3-ethylheptane 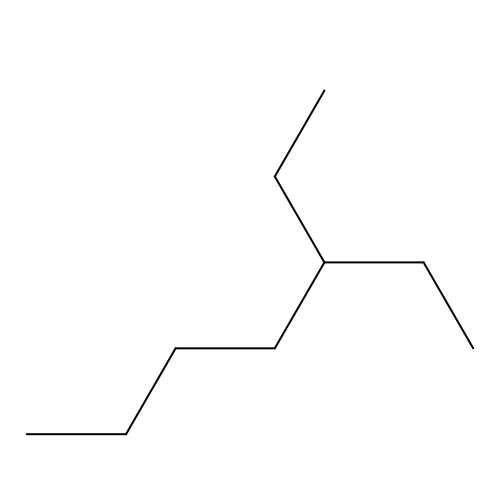| C9 H20 | PSVQKOKKLWHNRP-UHFFFAOYSA-N>[14x]DIYSRLLKDRIIMLGSQIDDNVANSIVSQLLFLQAQDSEKDIYLYINSPGGSVTAGFAIYDTIQHIKPDV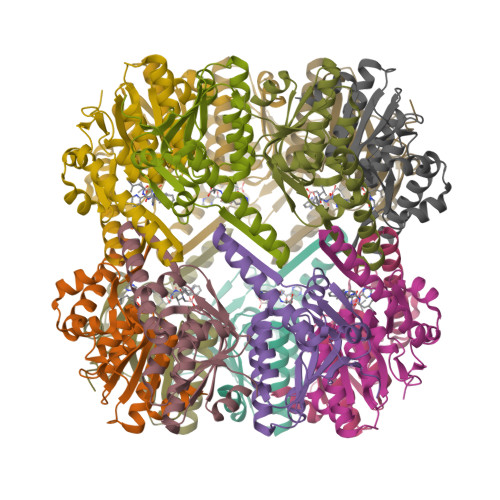QTICIGMAASMGSFLLAAGAKGKRFALPNAEVMIHQPLGGAQGQATEIEIAANHILKTREKLNRILSERTGQSIEKIQKDTDRDNFLTAEEAKEYGLIDEVMVPE> GPPDLGTDDDDKAMADIASDFPNNKETGEALLTPVDATASSHDGNGPDRLIDQDLTTRWSSAGDGEWAMLDYGSVQEFDAVQAS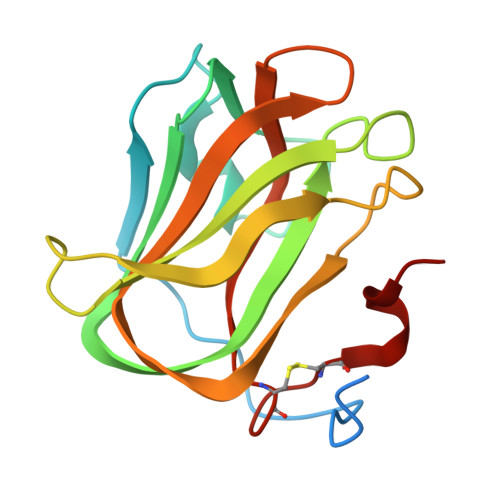FSKGNERQSKFDIQVSVDGETWTTVLENQLSSGKAIGLERFQFEPAVKARYVRYVGHGNTKNGWNSVTGLAAVNCSINACPASQIIT>MDSWLNMMLLCGLLLIASLQTTNAFRFRRSKSEMTHLETNIHSLQEHYKTRGTEWVSKSVFVPHLNQLNSKASCTCQALLLERMLNIYEELFQDMKSEHKEGRKDLDHLMDEVKKLRGNYKEEHKVWKELQEMN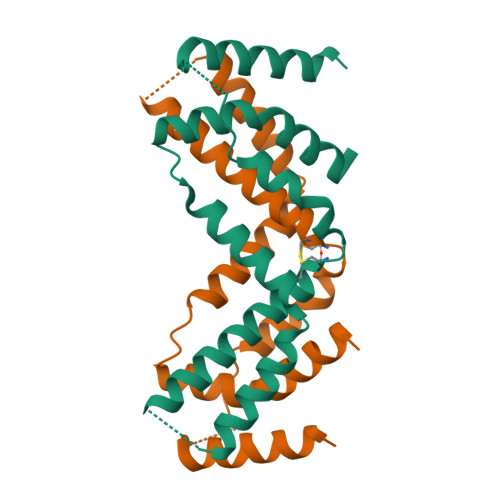SVKVKNGTIRGGALNDFLMVFDRASTEKHKKVQ[2x]Curli proteins are produced via dedicated and tightly regulated cellular processes, and their fibrils mediate host cell adhesion and invasion, lead to immune system activation, and scaffold bacterial communities known as biofilms. The two key players in curli fibril formation are CsgA and CsgB, the major and minor curli subunits, respectively. CsgA, a 151-residue protein, consists of five imperfect sequence repeats (R1-R5), defined by regularly spaced serine (Ser), glutamine (Gln) and asparagine (Asn) residues. The first and the last repeats (R1 and R5) form amyloid fibrils in isolation and are critical to CsgA seeding and nucleation by CsgB, while the other repeats (R2-R4) contain 'gatekeeper' residues that temper the amyloidogenicity of CsgA.

129TASNSS134 was selected as a control sequence as it was computationally predicted to be amyloidogenic but is located in a region not implicated in fibrillation. However, while 45LNIYQY50 (R1), 47IYQYGG52 (R1), and 137VTQVGF142 (R5) formed unbranched and elongated amyloid-like fibrils, the 129TASNSS134 (R4-R5 loop) segment formed scarce and more amorphous structures. The 129TASNSS134 segment from the R4-R5 loop did not bind ThT. Unlike the three spine segments that adopted tightly packed steric zipper architectures, 129TASNSS134 adopted an anti-parallel β-sheet structure lacking a dry interface between mated sheets. The packing of the β-sheets most closely resembled a class 8 steric zipper, with a truncated interface between the two facing β-sheets. In contrast, 129TASNSS134 does not contain any residues that have been shown to act as sequence determinants of CsgA fibrillation, and moreover, Ser133 is nonessential for fibrillation. Furthermore, in agreement with its atypical crystal structure, 129TASNSS134 formed scarce and more amorphous structures, and did not bind ThT. These observations demonstrated that not all segments that are predicted to have high aggregation propensities actually form steric zippers. The R1 segment 47IYQYGG52 and the control segment 129TASNSS134 showed a milder effect on the fibrillation rate of Aβ1–40.

> TASNSS>MSLSLKIALISQNENLLNLFPKLALEKNFIPITKTASLTRASKIAFGLQDEVDAIISRGATSDYIKKSVSIPSISIKVTRFDTMRAVYNAKRFGNELALIAYKHSIVDKHEIEAMLGVKIKEFLFSSEDE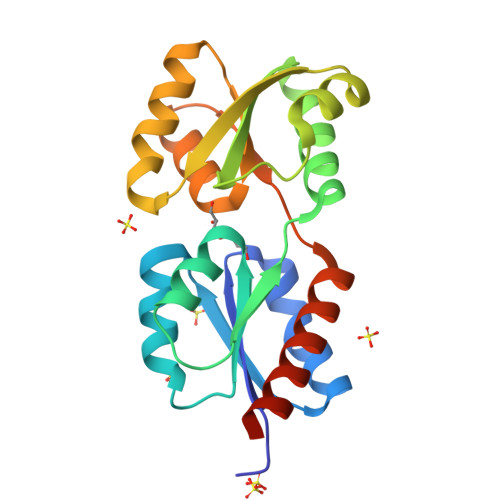ITTLISKVKTENIKIVVSGKTVTDEAIKQGLYGETINSGEESLRRAIEEALNLIEVRNEGHHHHHH[2x]>[4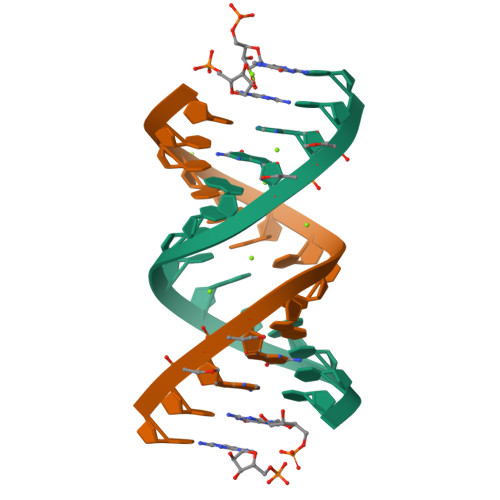x]NNAGACUUAAGUCU> VMTLPRIQDDLYLAVNGEWQAKTPIPPDKSVVSADSNLTDDIRQKLVADLSTMTKTAKTLPLQYAARLFAKANDQTRRQQLGIEPVRDRISFLMALTTLDQFRSAMPKLVADQYVLPISPYVDADMHDAEHNILNLGGPDTILPDAAMYNQEDAENAADLAAWSQMAAAMLAAVGFSQTDQTAYVEAAKRFDRRLADYVPANVDLAVDSTYDNPLSWQAFEDAAGYLGIPQAFATYMPQTPAKVNAVVPAYLPHLSKLLTPDNYSEWHAWMV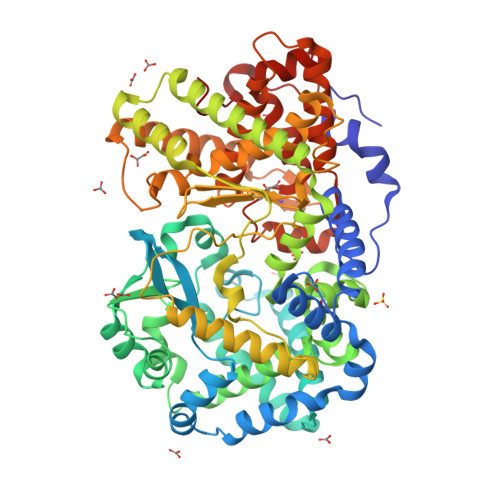INELLTCATYLSDDLRQLAGQYDRFLAGQPEASSWTKHAFGIANEYFDDVIGQYYGQTYFGADAKADVTAMVKQILAQYRVQLENNTWLSPATKQKAMRKLATMQVKMGYPARLFSLYDHLSVDVDDDLLTAILKLSAQTQAFWFKQLGQTVDRNQWNMPGHLVNASYDPLKNDITFPAGILQPPYYSLKWTRAENLGGTGATIGHEISHSFDNNGALYDEYGNLHNWWTPADKQAFDQLVKAMAAQFDGRDYEGVKVNGTLTVSENMADNAGMDVALALLGDQPDVKDLQAFFITYARSWATKMRPERAKTVLRQDVHAPATLRVNVPVQNFPAWYQAFNVQPQDGMYRQPQKRLTIWHQ> GAQVSTQKTGAHETGLNASGNSI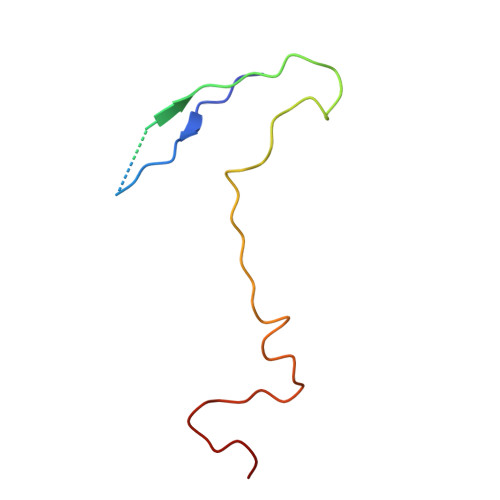IHYTNINYYKDAASNSANRQDFTQDPGKFTEPVKDIMIKSMPALN> GSHMRVTLSSKPQALATPNKEEHGKRKKKGKGLGKKRDPCLRKYKDFCIHGECKYVKELRAPSCICHPGYHGERCHGLS;> GADDVVDSSKSFVMENFSSYHGTKPGYVDSIQKGIQKPKSGTQGNYDDDWKGFYSTDNKYDAAGYSVDNENPLSGKAGGVVKVTYPGLTKVLALKVDNAETIKKELGLSLTEPLMEQVGTEEFIKRFGDGASRVVLSLPFAEGSSSVEYINNWEQAKALSVELEINFETRGKRGQDAMYEYMAQACAGNRVRRSVGSSLSCINLDWDVIRDKTKTKIESLKEHGPIKNKMSESPNKTVSEEKAKQYLEEFHQTALEHPELSELKTVTGTNPVFAGANYAAWAVNVAQVIDSETADNLEKTTAALSILPGIGSVMGIADGAVHHNTEEIVAQSIALSSLMVAQAIPLVGELVDIGFAAYNFVESIINLF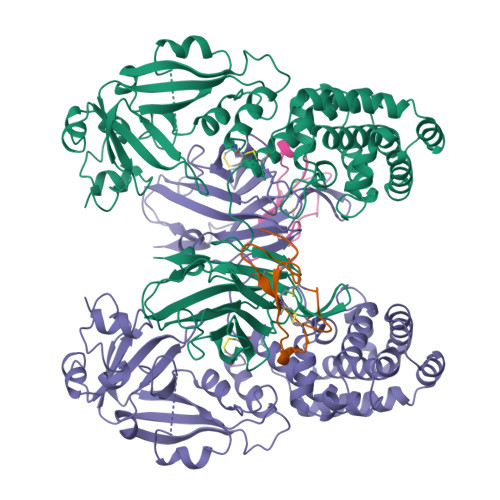QVVHNSYNRPAYSPGHKTQPFLHDGYAVSWNTVEDSIIRTGFQGESGHDIKITAENTPLPIAGVLLPTIPGKLDVNKSKTHISVNGRKIRMRCRAIDGDVTFCRPKSPVYVGNGVHANLHVAFHRSSSEKIHSNEISSDSIGVLGYQKTVDHTKVNSKLSLFFEIKS> DPLPFFPPLYLGGPEITTENCEREPIHIPGSIQPHGALLTADGHSGEVLQMSLNAATFL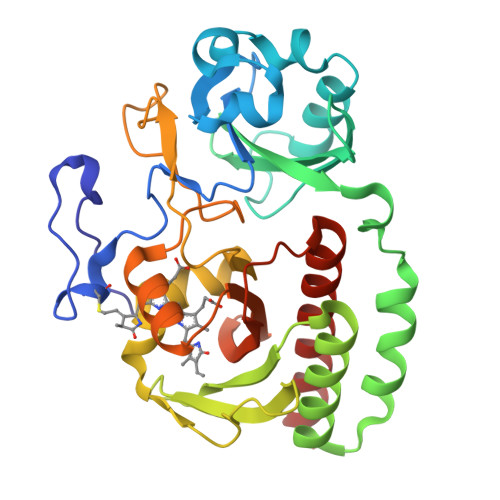GQEPTVLRGQTLAALLPEQWPALQAALPPGCPDALQYRATLDWPAAGHLSLTVHRVGELLILEFEPTEAWDSTGPHALRNAMFALESAPNLRALAEVATQTVRELTGFDRVMLYKFAPDATGEVIAEARREGLHAFLGHRFPASDIPAQARALYTRHLLRLTADTRAAAVPLDPVLNPQTNAPTPLGGAVLRATSPMHMQYLRNMGVGSSLSVSVVVGGQLWGLIACHHQTPYVLPPDLRTTLESLGRLLSLQVQVKEAH> MNLFRKKPIQLLMKESGAKGASLRKELGAFDLTMLGIGAIIGTGIFVLTGVAAAEHAGPALVLSFILSGLACVFAALCYAEFASTVPVSGSAYTYSYATFGELIAWILGWDLILEYGVASSAVAVGWSGYFQGLLSGFGIELPKALTSAYDPAKGTFIDLPAIIIVLFITFLLNLGAKKSARFNAVIVAIKVAVVLLFLAVGVWYVKPENWTPFMPYGFSGVATGAATVFFAYIGFDAVSTAAEEVRNPQRDMPIGIIVSLLVCTLLYIAVSLVLTGIVPYEQLNVKNPVAFALNYIHQDWVAGFISLGAIAGITTVLLVSMYGQTRLFYAISRDGLLPKVFARISPTRQVPYVNTWLTGAAVAVFAGIIPLNKL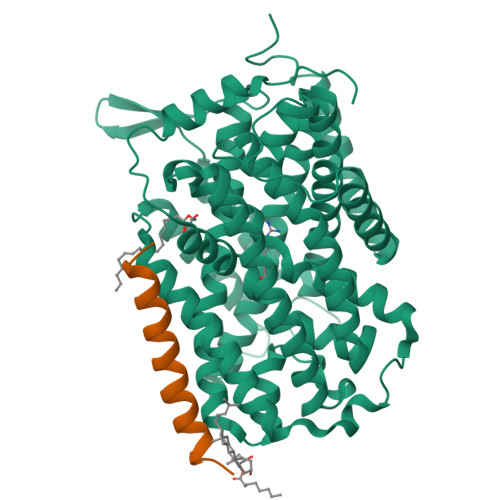AELTNIGTLFAFITVSIGVLVLRKTQPDLKRAFRVPFVPVVPILAVLFCGYLVLQLPAMTWIGFVSWLLIGLVIYFIYGRKHSELN;> MLGNMNVFMAVLGIILFSGFLAAYFSH>GSPEFSGREAKSRRRTSLPAPSPSSSNISLWNILRNNIGKDLSKVAMPVELNEPLNTLQRLCEELEYSELLDKAAQIPSPLERMVYVAAFAISAYASSYYRAGSKPFNPVLGETYECIREDKGFQFFSEQVSHHPPISACHAESRNFVFWQDVRWKNKFWGKSMEIVPIGTTHVTLPVFGDHFEWNKVTSCIHNILSGQRWIEHYGEIVIKNLHDDSCYCKVNFIKAKYWSTNAHEIEGTVFDRSGKAVHRLFGKWHESIYCGGGSSSACVWRANPMPKGYEQYYSFTQFALELNEMDPSSKSLLPPTDTRFRPDQRFLEEGNLEEAEIQKQRIEQLQRERRRVLEENHVEHQPRFFRKSDGSWVSNGTYLELRKDLGFSKLDHPVLW[2x]

Human ORP3 belongs to the oxysterol-binding protein (OSBP) family of lipid transfer proteins and is involved in lipid trafficking and cell signaling. ORP3 localizes to the ER-PM interfaces and is implicated in lipid transport and focal adhesion dynamics. The ORP3 ORD displays a helix grip β-barrel fold with a deep hydrophobic pocket which is conserved in the OSBP gene family. The ORP3 ORD has a central ligand-binding tunnel with a flexible lid covering the tunnel entrance.

The PI(4)P molecule was well ordered in the crystal structure with clear electron densities of the ligands. PI(4)P binds to the ORP3 ORD by inserting its two acyl chains into the hydrophobic tunnel. The phospho-inositol group of PI(4)P is recognized by the shallow basic pocket in the tunnel entrance. The conserved residues Lys829, Glu833, Arg836, and Arg837 from helix α8 make direct interaction with the phospho-inositol group. The 4-phosphate group makes hydrogen-bonds with the side-chains of the conserved His631 (β4-β5), His632 (β4- β5) and Arg837 (α8). The 1-phosphate group connecting the inositol ring and the glycerol moiety is hydrogen bonded to the conserved Lys603 (β2), Lys829 (α8) and the backbone amide atom of Met660 in the lid. The 5- and 6- hydroxyl groups of the inositol ring make direct hydrogen bonds with Gln836 (α8) and Glu833, respectively. The ORP3 ORD is unable to bind PI(4,5)P2 as the 5-phosphate group causes a steric clash with the side chains of the residues in the helix α8. The PI(4)P used in this structural study has the acyl chains of C8. Ligand modeling into the ORP3 ORD suggests that PI(4)P with various lengths of acyl chains up to C20 could be accommodated in the binding pocket.>GSIEIPMDLTQPPTITKQSVKDHIVDPRDNILIECEAKGNPAPSFHWTRNSRFFNIAKDPRVSMRRRSGTLVIDFRSGGRPEEYEGEYQCFARNKFGTALSNRIRLQVSKSPLWPKENLDPVVVQEGAPLTLQCNPPPGLPSPVIFWMSSSMEPITQDKRVSQGHNGDLYFSNVMLQDMQTDYSCNARFHFTHTIQQKNPFTLKVLTNNPYNDSSLRNHPDIYSARGVAERTPSFMYPQGTSSSQMVLRGMDLLLECIASGVPTPDIAWYKKGGDLPSNKAKFENFNKALRITNVSEEDSGEYFCLASNKMGSIRHTISVRVKAAPYWLDEPKNLILAPGEDGRLVCRANGNPKPTVQWMVNGEPLQSAPPNPNREVAGDTIIFRDTQISSRAVYQCNTSNEHGYLLANAFVSVLDVPPRMLSARNQLIRVILYNRTRLDCPFFGSPIPTLRWFKNGQGSNLDGGNYHVYENGSLEIKMIRKEDQGIYTCVATNILGKAENQVRLEVKDPTRIYRMPEDQVAKRGTTVQLECRVKHDPSLKLTVSWLKDDEPLYIGNRMKKEDDSLTIFGVAERDQGSYTCMASTELDQDLAKAYLTVLADQATPTNRLAAHHHHHH[2x]

Cell-surface expressed contactin 1 and neurofascin 155 control wiring of the nervous system and interact across cells to form and maintain paranodal myelin-axon junctions. Defining subfamily features are extracellular six N-terminal immunoglobulin-like domains (Ig), four fibronectin type III domains (FnIII) and posttranslational modifications, i.e., N-glycosylation at multiple sites and a C-terminal glycophosphatidylinositol (GPI)-membrane anchor. All four members are type I transmembrane proteins with six extracellular N-terminal Ig like domains, three to five FnIII domains, various predicted N-glycosylation sites, a single transmembrane spanning helix, and a ∼120 cytoplasmic region with a highly conserved ankyrin binding sequence. To address these questions, we structurally characterized the contactin 1 and neurofascin 155 interacting regions, i.e., Ig1–Ig6, individually and in complex.

Domains Ig5 and Ig6 interact head to tail and together make a V-turn with respect to Ig3–Ig4, giving the molecule a distinctive garden hoe like architecture. At the Ig4–Ig5 tip of the V-turn, neurofascin 155 N-terminal residues 23–31 wedge between these domains and interact intimately with both. The Ig4–Ig5 mediated V-turn is stabilized by extensive hydrophobic interactions, in which a central Phe466 of Ig5 is surrounded by Ile25, Ile27, Pro28 and Leu31 of the N-terminus, Ile358 and Leu437 of Ig4, and Val439, Leu444 and Ile 470 of Ig5. Conservation of the residues involved in the N-terminal, Ig4 and Ig5 interaction suggests the V-turn architecture of Ig4 and Ig5 is a shared feature of L1 family members. The 18-residue splice insert present in between domains of the Ig2–Ig3 unit in neurofascin 155, but absent in neurofascin 186, is for a large part unresolved in neurofascin 155 due to flexibility of this extended loop. At the center of the neurofascin 155 homodimerization interface, established by Ig2 domains with more modest Ig1 contributions, a super β sheet is formed by joining the G β-strands of both Ig2 domains. The dimerization interface overlaps with the binding site for contactin 1, suggesting that competition may exist between neurofascin 155 dimerization and contactin 1 binding. The Ig2–Ig3 unit combination hinges at its connections to Ig1 and Ig4 by a 17° rotation that bends the plane of the Ig1–Ig4 horseshoe. Despite the stabilizing role of the N-terminus, the Ig5–Ig6 combination swings parallel to the Ig1–Ig4 horseshoe by a 19° hinge at the Ig4–Ig5 connection. Glycans at Asn residues 316, 457 and 494 are juxtaposed in the space between the Ig1–Ig4 horseshoe and the Ig5–Ig6 combination and may limit the flexion between Ig4–Ig5 depending on the glycan composition.>[18x]MSKESSVAPTERVNIVYKPATGNAQEQVELPLKVLMLGDFTGQEDARPLEQRAPINVDKANFNEVMAQQNLKVTLTAADKLSADPNATMNVSLQFKNLNDFSPESVVNQVPELKKLLELRSALNALKGPLGNLPAFRKKLQALLADEDGRKALIKELGLTEETK;>MANETQTQKSTGVANDASLSLLDEILSEAKLKPKDEGYDVAKRGVQAFITEMLAPNRSEERVDKALVDAMIAEIDKRLSSQVNEILHAKEFQKLESSWRSLKFMVDRTDFRENTRVEMLNASKEDLQKDFEDAPEVTKSGLYKLVYSNEYGVFGGKPYGIISANYDFNVGPQDMELLRKCASVAAM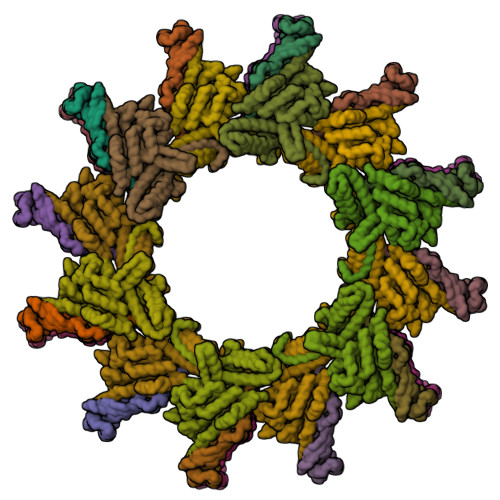AHAPFIGNAAPEVFGEESFLKLPDLKDLKSLFEGPQYARWHSFRESEDARYVGLALPRFLLRLPYGEKTVPVKAFNFTEDVVGHHERYLWGHASVALTSRVADSFAKFRWSPNIIGPQSGGAVENLPLHQYEAMGEIQTKIPTEVMLTERREFELSEEGFIGLVFRKDSDNAAFFSANSTQKPRFFGNTPEGKAAETNYRLGTQLPYMFIMTRLAHYIKVLQREQIGSWKEKSDLERELNHWLSQYISDMDDPAPAVRSRRPLRAARVVVEDVEGQPGWYRCSLQVRPHFKYMGASFTLSLVGKLDKE[18x]We previously showed that LJ0536, a cinnamoyl esterase purified from L. johnsonii N6.2, is active towards a variety of substrates including short acyl chain aliphatic esters and phenolic esters. The structure showed a canonical α/β fold characteristic of esterases, and the enzyme is dimeric. Two classical serine esterase motifs (GlyXSerXGly) can be recognized from the amino acid sequence, and the structure revealed that the catalytic triad of the enzyme is formed by Ser106, His225, and Asp197, while the other motif is non-functional. The structure revealed a prominent inserted α/β subdomain of 54 amino acids, from which multiple contacts to the aromatic acyl groups of the substrates are made.

The Ser106Ala-ethyl ferulate complex crystallized in two forms (Form I and Form II with a dimer and a single chain in the asymmetric units, respectively). The two ethyl ferulate crystal forms are nearly identical in structure. The root mean square deviation (RMSD) values of 244 Cα atoms of both chains of Form I onto Form II are 0.25 and 0.3 Å, respectively, and the dimer from Form II is essentially identical to the Form I dimer. In all three complexes, the substrates in the catalytic groove were oriented with the aromatic acyl moiety of the carbonyl group bound in the deepest part of the pocket. The opposite end of the ligands, on the far side of the ester moiety, such as the ethoxyl group of ethyl ferulate, rests on a more solvent-exposed area of the groove and has few interactions with the protein. The 3-methoxy group of ethyl ferulate or ferulic acid is accommodated by a small hydrophobic cavity formed by the benzyl moieties of Phe34 and Phe160, plus the Leu165 residue. In addition, there was relatively poor density for the alkoxyl group, perhaps due to the lack of direct interaction with the catalytic pocket.

>[2x]MGSSHHHHHHSSGRENLYFQGMATITLERDGLQLVGTREEPFGEIYDMAIIFHGFTANRNTSLLREIANSLRDENIASVRFDFNGHGDSDGKFENMTVLNEIEDANAILNYVKTDPHVRNIYLVGHAQGGVVASMLAGLYPDLIKKVVLLAPAATLKGDALEGNTQGVTYNPDHIPDRLPFKDLTLGGFYLRIAQQLPIYEVSAQFTKPVCLIHGTDDTVVSPNASKKYDQIYQNSTLHLIEGADHCFSDSYQKNAVNLTTDFLQNNNAF2'-deoxy-5'-O-[(R)-hydroxy{[(R)-hydroxy(phosphonooxy)phosphoryl]amino}phosphoryl]guanosine 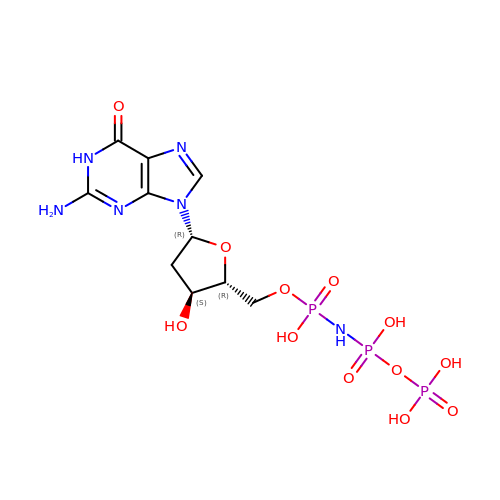| C10 H17 N6 O12 P3 | DWGAAFQEGIMTIA-KVQBGUIXSA-N> ATQKIAFSATRTINVPLRRDQTIRFDHV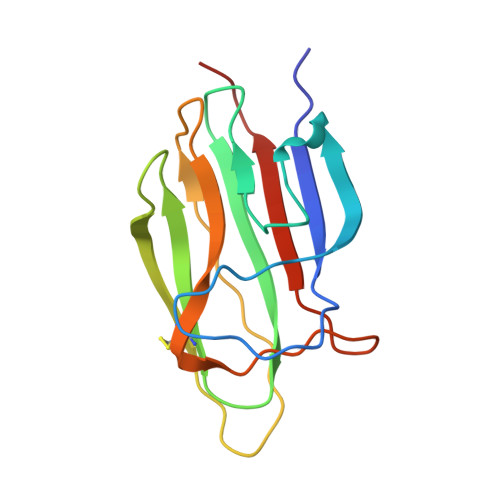ITNMNNNYEPRSGKFTCKVPGLYYFTYHASSRGNLCVNLMRGRERAQKVVTFCDYAYNTFQVTTGGMVLKLEQGENVFLQATDKNSLLGMEGANSIFSGFLLFPDMEA>[2x]MLSATQPLSEKLPAHGCRHVAIIMDGNGRWAKKQGKIRAFGHKAGAKSVRRAVSFAANNGIEALTLYAFS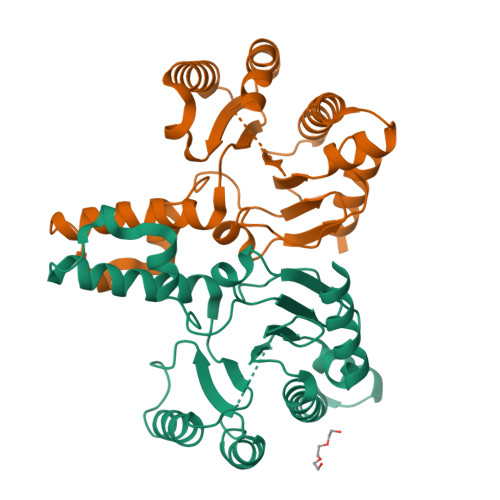SENWNRPAQEVSALMELFVWALDSEVKSLHRHNVRLRIIGDTSRFNSRLQERIRKSEALTAGNTGLTLNIAANYGGRWDIVQGVRQLAEKVQQGNLQPDQIDEEMLNQHVCMHELAPVDLVIRTGGEHRISNFLLWQIAYAELYFTDVLWPDFDEQDFEGALNAFANRERRFGGTEPGDETA> MRAVNWNKKEDDFSLMFWKQNIAQFWTEEEIAVSSDKNTWVQLSKEEQIAYK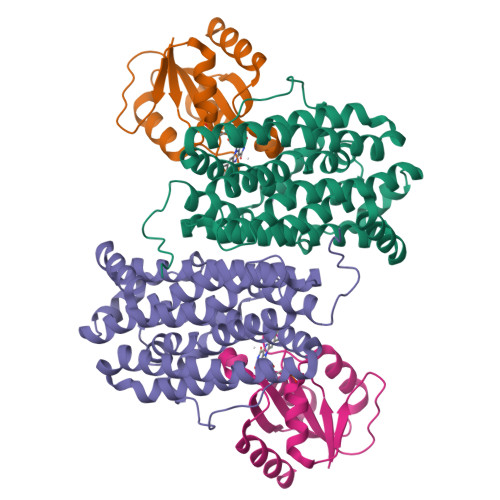RVLGGLTLLDTKQGGEGMPLVLVHLENLQAKSVLAFMGAMEEVHAKSYSHIFTTLATEEEIDDIFDWVDNHPLLEKKAGIITSYYRRLLKPEVTKKELYMAMVASVFLESYLFYSGFFYPLYLAGQGKLTASGEIINLIIRDESIHGVFVGILAQQIFAELSAEEQQEVQKETQELLMELYEIEMAYTEEIYTSIGLVEDVNRFVRYNANKGLMNLGLEPKFEEEEINPIVLNGLRTDTKNHDFFSVKGNGYVKATNVEKLADDDFVFNF;> MLVAYDSMTGNVKRFIHKLNMPAVQIDEDLVIDEDFILITYTTGFGNVPERVLDFLERNNEKLKGVSASGNRNWGDMFGASADKISTKYEVPIVSKFELSGTNNDVEYFKERVREIATH> GGGGGGMVGLLVEDTIDDQGWNRKAYEGLLNIHSNLDVDVVLEEGVNSEQKAHRRIKELVDGGVNLIFGHGHAFAEYFSTIHNQYPDVHFVSFNGEVKGENITSLHFEGYAMGYFGGMVAASMSETHKVGVIAAFPWQPEVEGFVDGAKYMNESEAFVRYVGEWTDADKALELFQELQKEQVDVFYPAGDGYHVPVVEAIKDQGDFAIGYVGDQADLGGSTILTSTVQHVD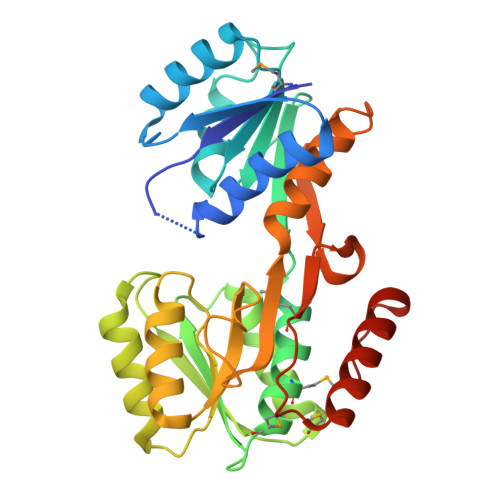DLYVLVAKRFQEGKLESGNLYYDFQDGVVSLGEFSSVVPDEVREQITDAISTYIQTGQFPHEEER> MSEIILTPKEQPEVPLEAPNIKPDVFAGKSIEEIKNIQIMHGNEVVKLGDFFEVSGEPADAPEDIKIIIDGDVYNTKRIGQEMTAGEIIVRGNVNMYVGAGMKGGKITVEGNAGSWAGQDMRGGEIEILGDAGDYVGSSYRGDWRGMSGGTITVHGNADNEIGEYMNGGKIIIKGDVNIMPGIHMNNGLIIIEG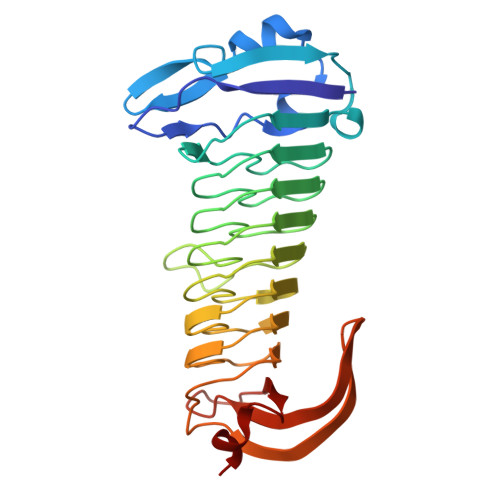NVVARAGGEMAGGTIVVKGMMQEFLAGFKYLGVEKDIEVDGEELPGAFYKFEGDHAIKGAKGIVYAAVGCNGHIAP The responsible exoribonuclease is Usb1, which removes nucleotides from the 3′ end of U6 and, in humans, leaves a 2′,3′ cyclic phosphate that is recognized by the Lsm2–8 complex. Usb1 is a member of the 2H phosphodiesterase superfamily of enzymes, which contain two vicinal active site HxS/T motifs that are essential for catalysis. We examine the structure and function of Usb1 from Kluyveromyces marxianus, which shares 25 and 19% sequence identity to the S. cerevisiae and Homo sapiens orthologs of Usb1, respectively. We find that the origin of CPDase activity is related to a loop structure that is conserved in yeast and forms a distinct penultimate (n – 1) nucleotide binding site.

Subsequent trials were performed with N-terminally truncated Usb1 by removing the first 58 amino acids (residues 59–275) that was designed to mimic the crystallizable S. cerevisiae and human orthologs of Usb1 (5,11,14). The structure of KmUsb1 was determined by single isomorphous replacement with anomalous scattering (SIRAS) methods and a uranyl acetate heavy atom derivative. The asymmetric unit contains three subunits, each of which is essentially identical in structure with an average alpha carbon pairwise r.m.s.d. of 0.63 Å for residues 61–275. Consistent with previously determined Usb1 structures, KmUsb1 retains the canonical 2H fold, with two conserved HxS motifs buried in the central cleft between the transit and terminal lobes in a very narrow channel that is just wide enough to accommodate single stranded, but not double stranded RNA. In addition, two glycerol molecules are bound in the catalytic pocket as high-occupancy ligands (calculated values are between 0.87 and 1.0), where one of the expected catalysts (His211) forms a hydrogen bond to a hydroxyl group of a glycerol molecule. The active site of KmUsb1 is similar to ScUsb1 as both have a 310-helix loop architecture in the n nucleotide binding pocket (residues 207–209 in KmUsb1) which is absent in HsUsb1. In contrast, this loop is much larger in both KmUsb1 and ScUsb1, with an overall positive charge and includes a 310-helix structure. The overall K. marxianus, S. cerevisiae and human Usb1 structures are highly homologous, although KmUsb1 more closely resembles ScUsb1 (the r.m.s.d. values are 3.1 Å for 182 aligned alpha carbon residues between KmUsb1 versus ScUsb1, and 4.1 Å for 159 aligned alpha carbon residues between KmUsb1 versus HsUsb1).

>MVAPVSKNIGFLFLELRLDSKQQQIMDLVLKGVNAVMDTHHRNSFEPLHRGKFGAMKPLHVSLSETMMFANESELEEKMGRIRQEIRALECKSVPVALSGGWLVYENFDASLQFLAVGLSEPARGRLKPVLSIVEKYKPRSPVSRQPVGLNNLHVSFGVAQNAYLQQDESVSRQRLDSLRNLVATEASDRLPLLRANLQFRCHELKAKVGTSVITLPL[3x]(3S,5R)-5-{[4-(2-chlorophenyl)-2,2-dimethyl-5-oxopiperazin-1-yl]methyl}-N-(3-methylbutyl)piperidine-3-carboxamide 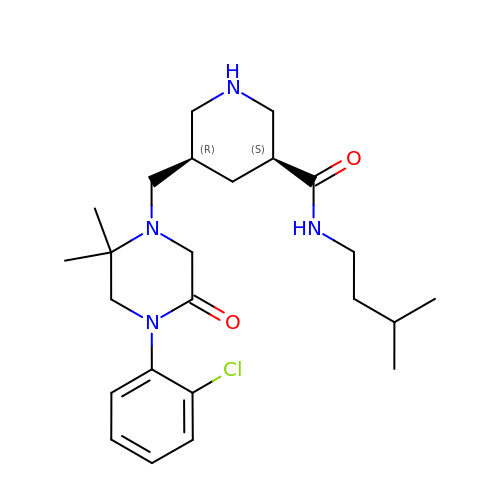| C24 H37 Cl N4 O2 | XGYKQWJDBJCEAW-MOPGFXCFSA-N> X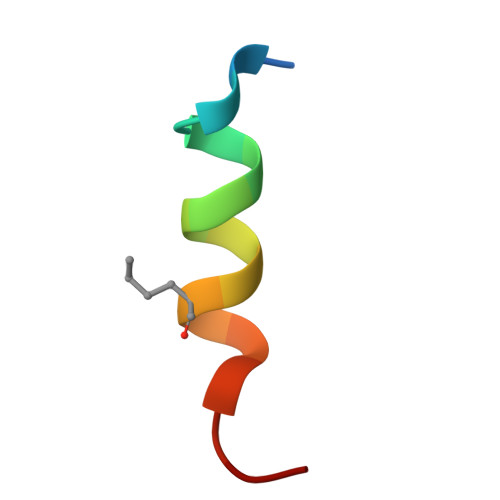LTFXEYWAQLLAAAAAA>[2x]MGSSHHHHHHSQDLEVLFQGPHMAFEKPLRKLTFADLLQATNGFHNDSLIGS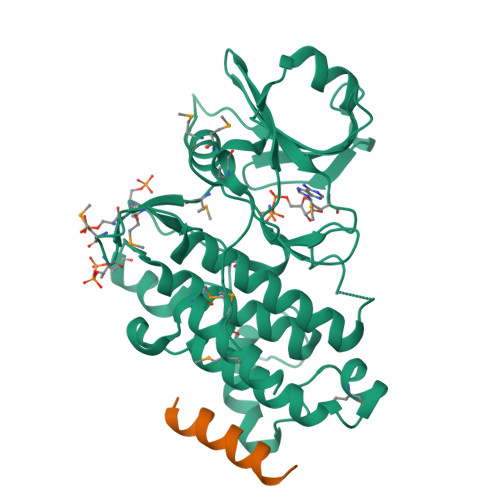GGFGDVYKAILKDGSAVAIKKLIHVSGQGDREFMAEMETIGKIKHRNLVPLLGYCKVGDERLLVYEFMKYGSLEDVLHDPKKAGVKLNWSTRRKIAIGSARGLAFLHHNCSPHIIHRDMKSSNVLLDENLEARVSDFGMARLMSAMDTHLSVSTLAGTPGYVPPEYYQSFRCSTKGDVYSYGVVLLELLTGKRPTDSPDFGDNNLVGWVKQHAKLRISDVFDPELMKEDPALEIELLQHLKVAVACLDDRAWRRPTMVQVMAMFKEIQAGSGIDSQSTIRSIEDGGFST;>[2x]STMEELQAAIQAAIAHCKNSY> MHHHHHHHHENLYFQGSETPAEPKLPVVVEAHQVDTFDVPGVFYENHPHEPHLSGMNEYNQLYQQSINDPDTFWARMARDLITFEKDFDKTHIGTLEGGDNAWFVGGRLNASFNCVDRHAMRDPNKV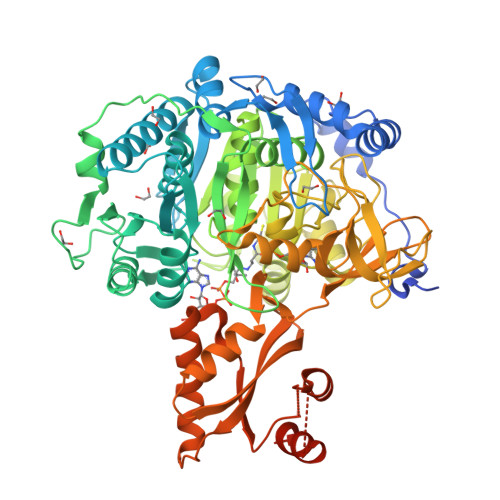AIIYEADEPGHGRSITYAELLKEVSRLAWVMKSQGVRKGDTVAIYLPMIPEAIFALLACARIGAIHSVVFAGFSSDSLRDRTLDARSKFIITTDEGKRGGKVIGTKKIVDEALKQCPDVTNCLVFKRTGADVPWTKGRDLWWHEEVDKYPNYLPAESMDSEDPLFLLYTSGSTGKPKGVMHTTAGYLVGAAATGKYVFDIHPADRFFCGGDVGWITGHTYVVYAPLLLGCTTVVFESTPAYPNFSRYWDVIEKHKVTQFYVAPTALRLLKRAGDHHINHEMKDLRILGSVGEPIAAEVWKWYHEVVGKRQAHIVDTYWQTETGSHVITPLGGITPTKPGSASLPFFGIDPVILDPVTGAEIPGNDVEGILAFRKPWPSMARTVWGDHKRYMDTYLNVYKGFYFTGDGAGRDHEGYYWIRGRVDDVVNVSGHRLSTAEIEAALIEHHCVAEAAVVGVPDPLTGQAVHAFVALKSGNDNREQLQKELIMQVRKSIGPFAAPKVVFVIDDLPKTRSGKIMRRILRKILSGEEDSLGDISTLSDPSVVNKIIDTFHEWKKAMAAAAAAAAAVSATAPPNSTTG Two enzymes, peptidylglycine α-hydroxylating monooxygenase (PHM; EC 1.14.17.3) and peptidyl-α-hydroxyglycine α-amidating lyase (PAL; EC 4.3.2.5) working sequentially are the only proteins known to catalyze this reaction. PHM, a two Cu enzyme, catalyzes the stereospecific hydroxylation of the glycine Cα of peptidylglycine substrates. The two copper atoms in PHM, CuH, and CuM (located in the N- and C-subdomains, respectively), each use a single reducing equivalent from ascorbate to catalyze the reduction of molecular oxygen for the hydroxylation of the Cα of glycine at the carboxy-terminus of the peptide substrate. Crystallographic data on apo wild-type PHM and on several crystal forms of three CuH mutants (H107A, H108A, and H172A) presented here show that the copper ions are required not only for the catalytic steps but also for substrate binding and for locking the overall conformation of PHM in a configuration that is catalytically active.

The situation is different for the crystals obtained in the presence of 1–3 mM citrate: they diffract to 2.5 Å, the space group and cell dimensions are different from those of the wild-type and contain two identical molecules in the asymmetric unit with bound citrate. Neither molecule contains copper in the CuH site. When the N-subdomain of the H108A-PHM-cit structure is aligned with that of wild-type PHM, the C-subdomain displays a rotation of ~18° toward the N-subdomain, compared to its position in the wild-type PHM structure. As a consequence of this hinge movement, several secondary elements of the C-subdomain move as much as 15 Å closer to the N-subdomain. These changes result in a complete reorganization of the coordination of the copper in CuM. The two histidines, His 242 and His 244, remain coordinated to the copper, but Met 314 and the fourth ligand in wild-type PHM (a water molecule) do not bind to the ion. Of the two vacated Cu2+ coordination positions, one is occupied by the 2-carboxylate of citrate, and the other, surprisingly, by the Nε of His 107, originally a copper ligand of the CuH site. In the wild-type PHM structure, the distance between His242 Nε and His107 Nε is 11.7 Å, while it is 3.9 Å in the H108A-PHM-cit structure. The arrangement of subdomains in the DBH-cat of molecule A (closed) is highly similar to that of the H108A-PHM-cit structure (RMSD 1.19 Å for 195 Cα), including the position of the single copper ion of each structure (difference in position of the copper atom in the two aligned structures <1.6 Å). However, the fact that this conformation was only seen in structures with a single copper ion (H108A-PHM-cit and hDBH chain A) is more compatible with the conclusion that having two bound coppers has an important structural role: locking PHM (and probably DBH) in the catalytically competent conformation.

>[2x]NECLGTIGPVTPLDASDFALDIRMPGVTPKESDTYFCMSMRLPVDEEAFVIDFKPRASMDTVHAMLLFGCNMPSSTGSYWFCDEGTCTDKANILYAWARNAPPTRLPKGVGFRVGGETGSKYFVLQVHYGDISAFRDNHKDCSGVSVHLTRVPQPLIAGMYLMMSVDTVIPPGEKVVNADISCQYKMYPMHVFAYRVHTHHLGKVVSGYRVRNGQWTLIGRQNPQLPQAFYPVEHPVDVTFGDILAARCVFTGEGRTEATHIGGTSSDEMCNLYIMYYMEAKYALSFMTCTKNVAPDMFRTIPAEANIPIPV>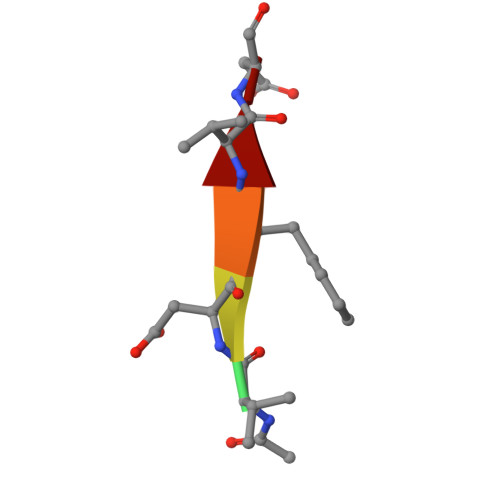 XVDFVD>[2x]DPTQFEERHLKFLQQLGKGNFGSVEMCRYDPLQDNTGEVVAVKKLQHSTEEHLRDFEREIEILKSLQHDNIVKYKGVCYSAGRRNLKLIMEYLPYGSLRDYLQKHKERIDHIKLLQYTSQICKGMEYLGTKRYIHRDLATRNILVENENRVKIGDFGLT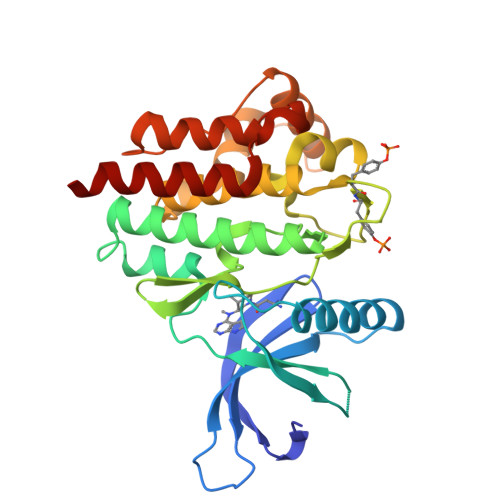KVLPQDKEYYKVKEPGESPIFWYAPESLTESKFSVASDVWSFGVVLYELFTYIEKSKSPPAEFMRMIGNDKQGQMIVFHLIELLKNNGRLPRPDGCPDEIYMIMTECWNNNVNQRPSFRDLALRVDQIRDQMAG> GPLGSGRPMLSTDNFKKIKLRDISLEDAIKASNYEEINNKVTDKKMAHQALAYSLGNKKADIALYLLSKFNFTKQDV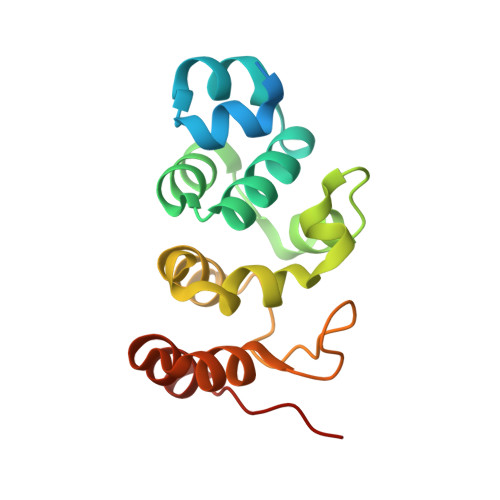AEMEKMKNNRYCNLYDVEYLLSKDGANYKVLEYFINNGLVDVNKKFQKVNSGDTMLDNAMKSKDSKMIDFLLKNGAILGKRFEI>[2x]MSLG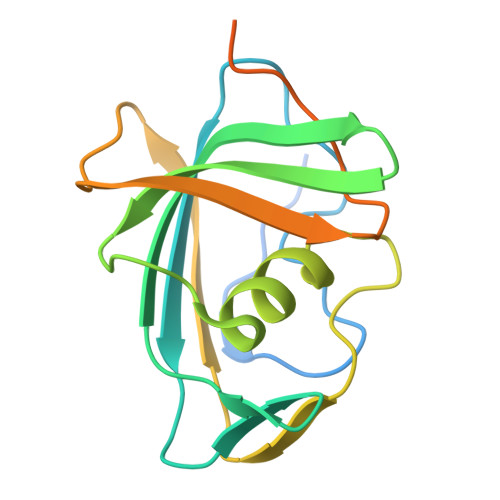QSDLHIDPTQFIMYSGTISNGISYVNQAPSCGTVLSLKFTPGNSSLIENLHIEPYKVEVLKIEHVGDVSRATLLSDIVSLSTAQKKLLLYGFTQPGVQGLTGDVVSVETKRIPTPTQTNLLTIEDSIQCFTWDMNCANARSTNQDSRLIIYEQEDGRSHHHHHH;> GAAG> 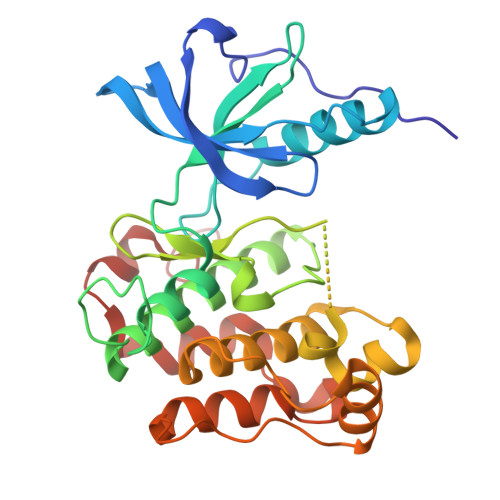VFPSSVYVPDEWEVSREKITLLRELGQGSFGMVYEGNARDIIKGEAETRVAVKTVNESASLRERIEFLNEASVMKGFTCHHVVRLLGVVSKGQPTLVVMELMAHGDLKSYLRSLRPEAENNPGRPPPTLQEMIQMAAEIADGMAYLNAKKFVHRNLAARNCMVAHDFTVKIGDFGMTRDIYETDYYRKGGKGLLPVRWMAPESLKDGVFTTSSDMWSFGVVLWEITSLAEQPYQGLSNEQVLKFVMDGGYLDQPDNCPERVTDLMRMCWQFNPNMRPTFLEIVNLLKDDLHPSFPEVSFFHSEENK> XTA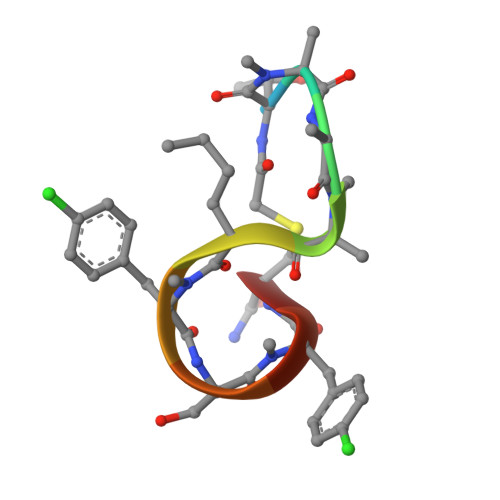AALFSFAX[6-(3-methoxyphenyl)-1-benzofuran-3-yl]acetic acid | C17 H14 O4 | 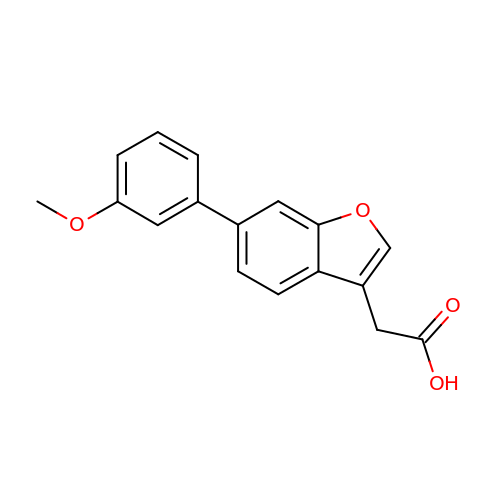BYTREUVWMDHJCQ-UHFFFAOYSA-N5-azaniumylpentylazanium | C5 H16 N2 | 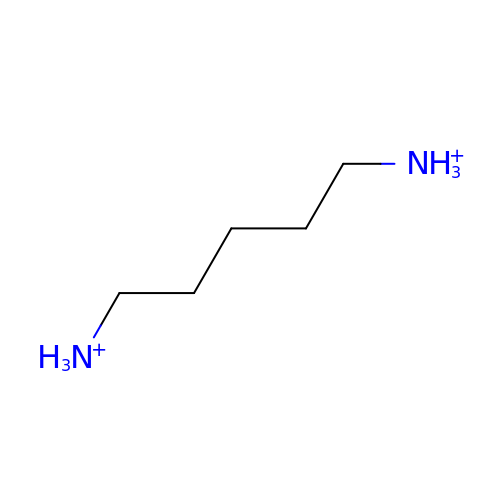VHRGRCVQAFMJIZ-UHFFFAOYSA-P>AIIRKNVNSLTPSDIKELRDAMAKVQADTSDNGYQKIASYHGIPLSCHYENGTAYACCQHGMVTFPNWHRLLTKQMEDALVAKGSHVGIPYWDWTTTFANLPVLVTEEKDNSFHHAHIDVANTDTTRSPRAQLFDDPDKGDKSFFYRQIALALEQTDFCDFEIQFEIGHNAIHSWVGGSSPYGMSTLHYTSYDPLFYLHHSNTDRIWSVWQALQKYRGLPYNTANCEINKLVKPLKPFNLDTNPNAVTKAHSTGATSFDYHKLGYDYDNLNFHGMTIPELEEHLKEIQHEDRVFAGFLLRTIGQSADVNFDVCTKDGECTFGGTFCILGGEHEMFWAFDRLFKYDITTSLKH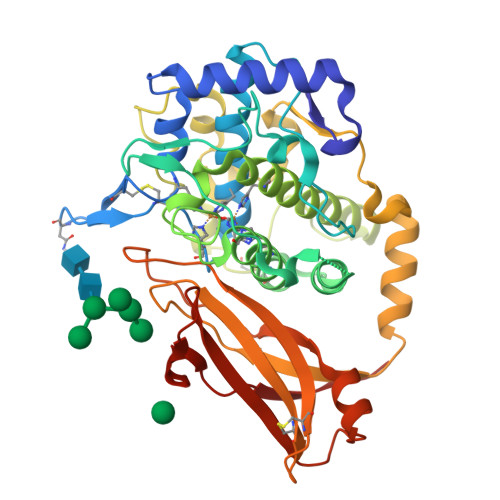LRLDAHDDFDIKVTIKGIDGHVLSNKYLSPPTVFLAPAKTTH[2x]> KVEQAVETEPEPELRQQTEWQSGQRWELALGRFWDYLRWVQTLSEQVQEELLSSQVTQELRALMDETMKELKAYKSELEEQLTPVAEETRARLSKELQAAQARLGADMEDVRGRLVQYRGEVQAMLGQSTEELRVRLASHLRKLRKRLLRDADDLQKRL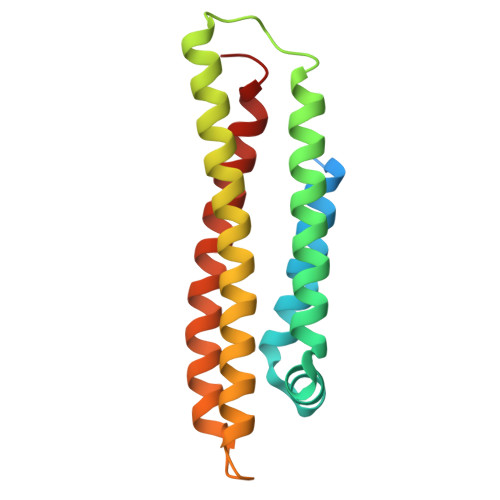AVYQAG> GPTEKAAVKKMAKA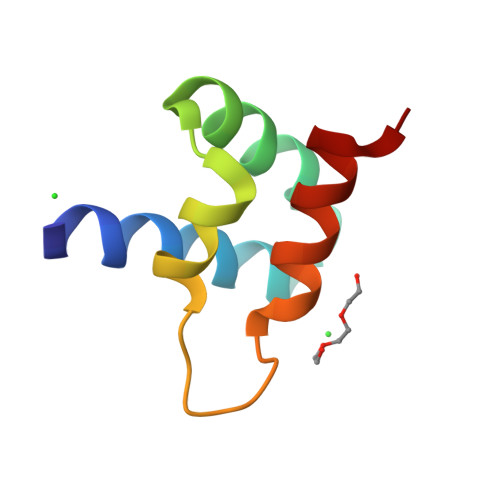IMADPSKADDVYQKWADKGYTLTQLSDFLKSKTRGKYDRVYNGYMTYRDYV>[2x]SMTDLLSAEDIKKAIGAFTAADSFDH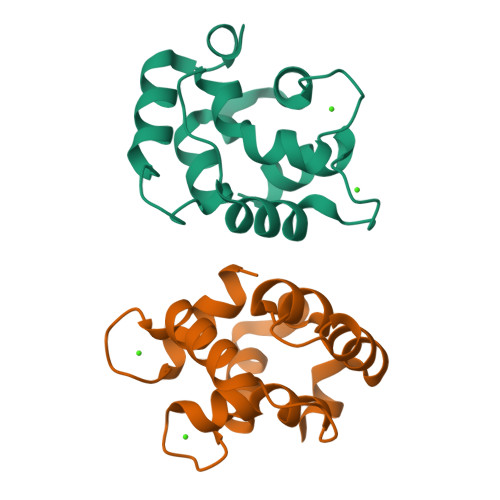KKFFQMVGLKKKSADDVKKVFHILDKDKSGFIEEDELGSILKGFSSDARDLSAKETKTLMAAGDKDGSGKIEVEEFSTLVAES> GAMEPSAPKELKFGDITKDSVHLTWEPPDDDGGSPLTGYVVEKREVSRKTWTKVMDFVTDLEFTVPDLVQGKEYLFRVCARNKCGPGEPAYVDEPVNMSTPATVPDPPENVKWRDRTANSIFLTWDPPKNDGGSRIKGYIVERCPRGSDKWVACGEPVAETKMEVTGLE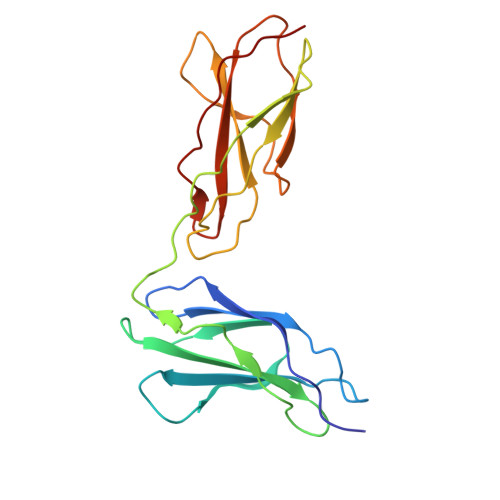EGKWYAYRVKALNRQGASKPSRPTEEIQAV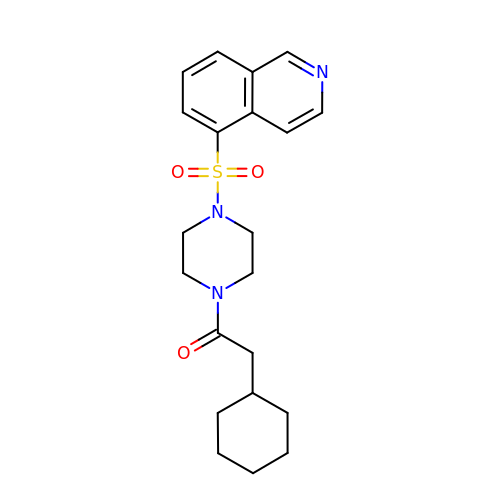2-cyclohexyl-1-{4-[(isoquinolin-5-yl)sulfonyl]piperazin-1-yl}ethan-1-one | C21 H27 N3 O3 S | CUMYYEWYWPAOFL-UHFFFAOYSA-N> MGHHHHHHENLYFQGHMASMNRTLTREQVLALAEHIENAELNVHDIGKVTNDFPEMTFADAYDVQWEIRRRKEARGNKIVGLKMGLTSWAKMAQMGVET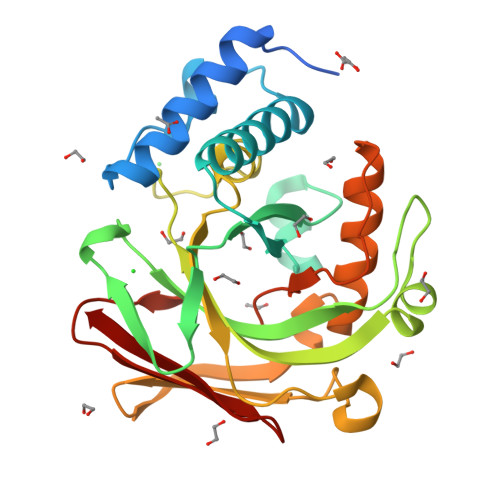PIYGFLADYFSVPDGGVVDCSKLIHPKIEAEISVVTKAPLHGPGCHLGDVIAAIDYVIPTVEVIDSRYENFKFDPISVVADNASSTRFITGGRMASLEEVDLRTLGVVMEKNGEVVELGAGAAVLGHPLSSVAMLANLLAERGEHIPAGTFIMTGGITAAVPVAPGDNITVRYQGLGSVSARFI>TLLISEVLKTSKQYLSVLAQVVDIQSSDKNIRLKICDNSCNQELKVVIFPDLCYEWRDKFSINKWYYFNEFVRQIYNDEVQLKNNIHSSIKESDDQRKVI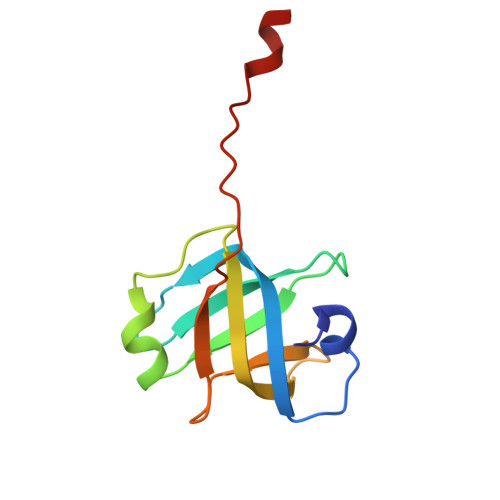TYNQEQGVF[2x]>GIDPFTMFEEINVVRAAELHRRDRFDPVPQLRSLMAEGPLTTLGTEESPGGRTAWLATGYDEIRQVLSSDDFSARLLYGGTAAGITWPGFLTQYDPPEHTRLRRMVAPAFAVRRMQKFQPQVERVVQDSLDAIEALGGPVDFVPRFGWSVATTATCDFLGIPRDDQADLARSLHASRTERSGKRRTAAGNKFMTYMNKMTARTRRDPGDDMFGVVVREYGDEITDAELTGVAAFVMGAGADQVARFLAAGAWLMADDPEQFALLREKPDTVPD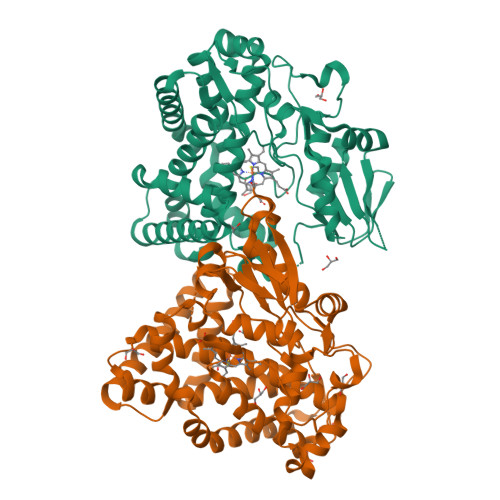WLDEVIRYLTTDEKTHPRVATDDVRIGDHLIKAGDTVTCSLLAANRRNFPRPEDRFDITRVRPEHLAFGHGIHHCLGRSLAELVFRTAIPALAHRFPTLRLAEPHREIRLGPPPFDVEALLLDW[2x]>SNAMRETFEIGEIVTGIYKTGKYIGEVTNSRPGSYVVKV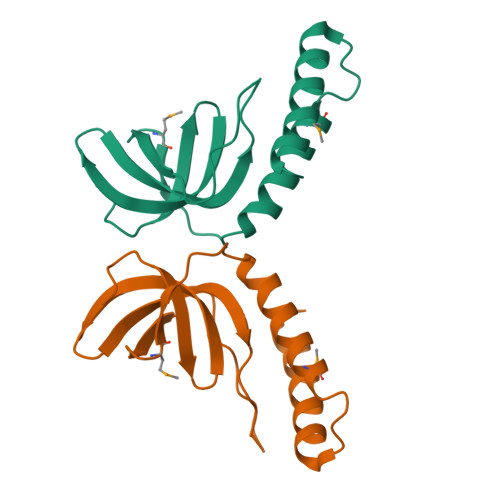LAVLKHPVQGDLHNVKQANVPFFHERRALAFREQTNIPEQMVKKYEGEIPDYTESLKLALETQMNSFSEDDSPFAERSLETLQQLKKDYKL[2x]>MRGSHHHHHHGSSTRSTGVENSGAGPTSFKTMKVIDPQHSDKPNVLILGSGWGAISFLKHIDTKKYNVSIISPRSYFLFTPLLPSAPVGTVDEKSIIEPIVNFALKKKGNVTYYEAEATSINPDRNTVTIKSLSAVSQLYQPENHLGLHQAEPAEIKYDYLISAVGAEPNTFGIPGVTDYGHFLKEIPNSLEIRRTFAANLEKANLLPKGDPERRRLLSIVVVGGGPTGVEAAGELQDYVHQDLRKFLPALAEEVQIHLVEALPIVLNMFEKKLSSYAQSHLENTSIKVHLRTAVAKVEEKQLLAK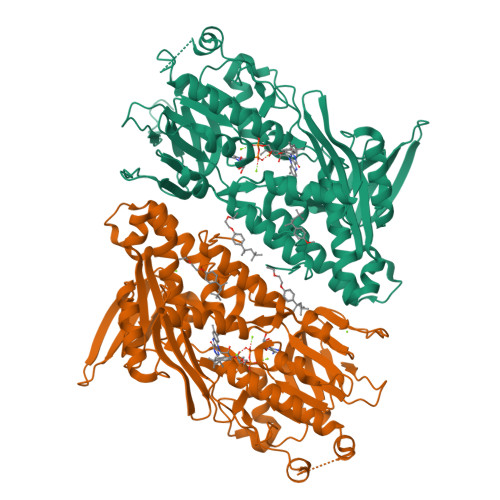TKHEDGKITEETIPYGTLIWATGNKARPVITDLFKKIPEQNSSKRGLAVNDFLQVKGSNNIFAIGDNAFAGLPPTAQVAHQEAEYLAKNFDKMAQIPNFQKNLSSRKDKIDLLFEENNFKPFKYNDLGALAYLGSERAIATIRSGKRTFYTGGGLMTFYLWRILYLSMILSARSRLKVFFDWIKLAFFKRDFFKGL[2x]> MLPNTKLHNTIFSETRKFTRESFKEIEHLTARLANDSVARHDFLFNTSIALISDYSGEDSNGNQLQATITIPNEIINPKEYDPSDYPLAEDESFFKQGHKYDYLVTFRAGSLTNTYEPKTKMYKLHAALDKLMHVRQRKSRFADLWRELCAVIASLDVWYQTTNYPLRTYVKLLFHRGDEFPFYESPSQDRIIFNDKSVASILPTFVYTCCQVGTAIMSGILTHVESIVAMNHFLHCAKDSYIDEKLKIKGIGRSWYQEALHNVGQATVPVWSQFNEVIGHRRKSTSEPHFVSSTFISLRAKRAELLYPEFNAYINRAIQLSKTQNDVANYYAACRAMTNDGTFLATLTELSLDAAVFPRIEQRLVTRPAVLMSNTRHESLKQKYTNGVGSIAQSYLSSFTDEIAKRVNGIHHDEAWLNFLTTSSPGRKLTEIEKLEVGGDVAAWSNSRIVMQAVFAREYRTPERIFKSLKAPIKLVERQQSDRRQRAISGLDNDRLFLSFMPYTIGKQIYELNDNAAQGKQAGNAFDIGEMLYWTSQRNVLLSSIDVAGMDASVTTNTKDIYNTFVLDVASKCTVPRFGPYYAKNMEVFEVGKRQSQVRYVNAAWQACALEAADSQTSTSYESEIFGQVKNAEGTYPSGRADTSTHHTVLLQGLVRGNELKRASDGKNSCLATIKILGDDIMEIFQGSESDTYDHAMSNANILNESGFATTAELSQNSIVLLQQLVVNGTFWGFADRISLWTREDTKDIGRLNLAMMELNALIDDLVFRVRRPEGLKMLGFFCGAICLRRFTLSVDNKLYDSTYNNLSKYMTLIKYDKNPDFDSTLMSLILPLAWLFMPRGGEYPAYPFERRDGTFTEDESMFTARGAYKRRLLYDVSNIREMIQQNSMALDDDLLHEYGFTGALLLIDLNILDLIDEVKKEDISPVKVSELATSLEQLGKLGEREKSRRAASDLKIRGHALSNDIVYGYGLQEKIQKSAMATKETTVQSKRVSSRLHDVIVAKTRDYKISTIPADALRLHEFEVEDVTVDLLPHAKHTSYSSLAYNMSFGSDGWFAFALLGGLDRSANLLRLDVASIRGNYHKFSYDDPVFKQGYKIYKSDATLLNDFFTAISAGPKEQGILLRAFAYYSLYGNVEYHYVLSPRQLFFLSDNPVSAERLVRIPPKYYVSTQCRALYNIFSYLHILRSIANNWGKRLKMVLHPGLIAYVRGTSQGAILPEADNV;> MFAIDPLKHPKLYEEYGLYLRPHQINQEIKPTTIKKKELAPTIRSIKYASLIHSMLAKHAARHNGTLINPRMYADMITLGNTKVTVTKGTPKAQIDTLKMNGLTVVSKSRRNNKKKPVSDTTASTDETTDDVVTYKALTEMSTLVESFRLPSGLTLIVFDDEKYQSLIPDYINQLITYTQPHIIPTWQ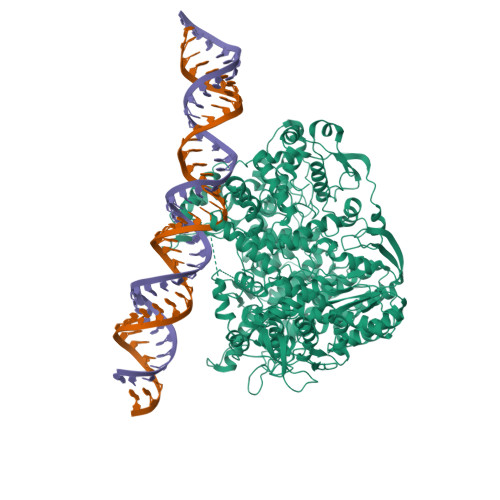GITDFSDTYLRSYFKRPFELTASNLAVPQKHNLSPITRSIFNNTGREDAIIRKLYGYGEYVFIKYEGCLITWTGLYGAVTMMVNLPKRDLGLDVGDDFLKEYKKLLFHGVITDAIPSGISAKSTVMRISPHKMMNPSGGALAVLSKYIEAVVSTNVINATLVVYAEKGAGKTSFLSTYAQQLSLASGQIVGHLSSDAYGRWLAKNKDVEEPSFEYDYVLSLDTDDNESYYEQKASELLTSHGISELSQYELLSVRRKVKMMNEMDEILIAQLDNANTHSERNFYYMVSTGKNTPRTLIVEGHFNAQDATIARTDTTILLRTINDTTQAMRDRQRSGVVQLFLRDTYYRLLPSLHTTVYPFEMLESIKRWKWVH> QINDLPVCQSSRRTIHSRPSGKRLFLTGATGFLGTHILHQLLVDNDVSIVYVLARAPCPRKGLARIIQAARLARWWRNDYRRLIQVWPGDLSQPHLGLADEHWETLSGTESSLNSSIGAVDAIIHC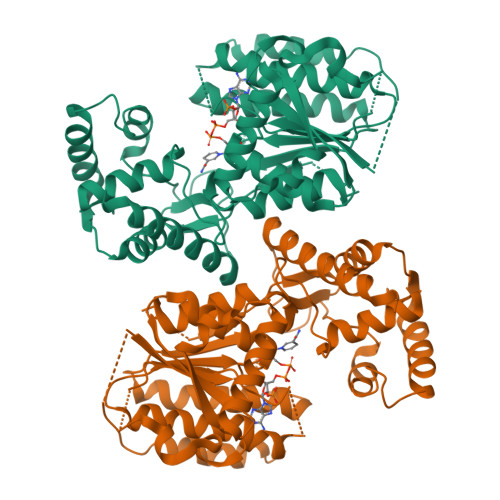GAVIHWGYDYDTLEAANVRSTFDILQCLNRSPTPIALTYISALIPGDAALATTDTDNHPSMSNGHAVFPPIELTDGYTQTKFASEQLIGAFSARHKAHSLTIVRPGFMIGPVSNAVANGDDLLWRVVTTAMTTCSYNSDESDNWLFVAAVDWVASLIIHETLHARPSSHSVNDNANPLAPSAKAVSIGDGLNMSDFWKAIMLGLGRDLIPSSSQRWMDTVEQQVNEVGTSHPLWPLMGFLRASGGCLGVAPTDPLPVPIYQPPSLTNMIRQAVVRNAEYLASLEDLAASTMLFKRRNKVALGNGLINS> RKLCS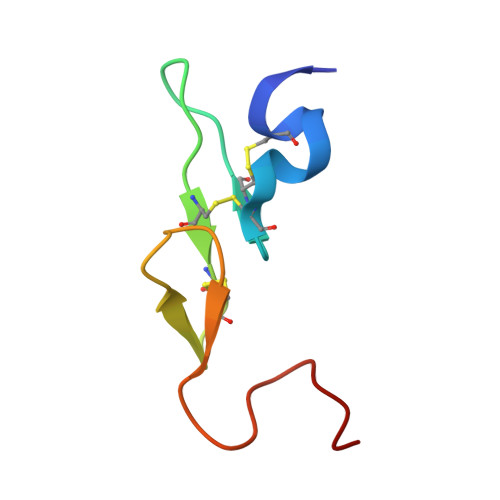LDNGDCDQFCHEEQNSVVCSCARGYTLADNGKACIPTGPYPCGKQTL> MGAEKKLFLKALKEKFEEDPKEKYTKFYVFGGWRQSARKREFVEAAEKLAEKRGGIPFYNPDIGVPLGQRKLMPYKLSGTDYIVEGDDLHFMNNAAMQQFWDDIRRTVIVGMDTAHAVLEKRLGVEVTPETINEYMETINHALPGGAVVQEHMVEVHPALAWDCYAKIFTGDDELADEIDKKFLIDINKLFPEEQAEQLKAAIGKRTYQVSRVPTLVGRVCDGGTIARWSAMQIGMSFITAYKLCAGEAAIADFSYAAKHADVIQMGTLLPARRARGPNEPGGIPFGILADVVQTTRVSDDPVEQSLEVVASGAMLYDQIWLGSYMSGGVGFTQYATASYTDDILDDFSYYGYDYVEK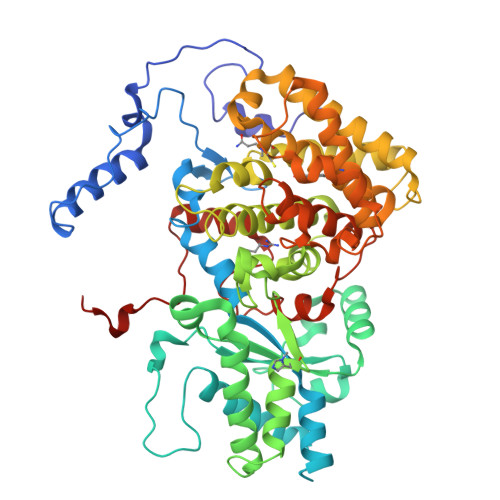KYGICGAKPTMDVVEDIATEVTLYALECYDEFPALLEDHFGGSQRAAVAAAASGISVCMATGNSNAGLNGWYLSQILHKEYHSRLGFYGYDLQDQCGASNSLSIRNDESSPLELRGPNYPNYAMNVGHQGEYAGITQAAHSARKDAFALNPLIKVAFADPSLVFDFSHPRKEFARGALREFEPAGERDPIIPAH> GSPGISGGGGGESGLTPLHVASFMGHLPIVKNLLQRGASPNVSNVKVETPLHMAARAGHTEVAKYLLQNKAKVNAKAKDDQTPLHCAARIGHTNMVKLLLENNANPNLATTAGHTPLHIAAREGHVETVLALLEKEASQACMTKKGFTPLHVAAKYGKVRVAELLLERDAHPNAAGKNGLTPLHVAVHHNNLDIVKLLLPRGGSPHSPAWNGYTPLHIAAK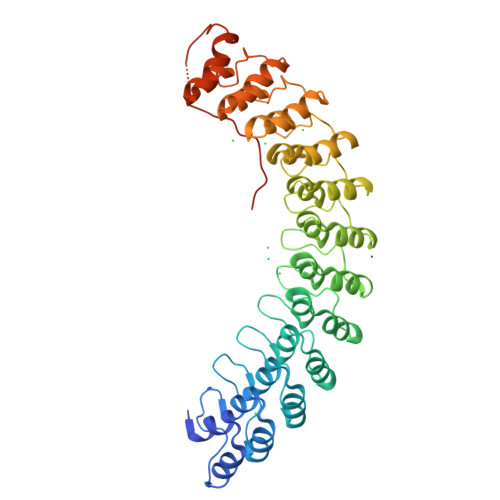QNQVEVARSLLQYGGSANAESVQGVTPLHLAAQEGHAEMVALLLSKQANGNLGNKSGLTPLHLVAQEGHVPVADVLIKHGVMVDATTRMGYTPLHVASHYGNIKLVKFLLQHQADVNAKTKLGYSPLHQAAQQGHTDIVTLLLKNGASPNEVSSDGTTPLAIAKRLGYISVTDVLKVVTDETSFVLVSDKHRMSFPETVDEILDVSEDEGEELISF> KETAAAKFERQHMDSSTSAASSSNYCNQMMKSRNLTKDRCKPVNTFVHESLADVQAVCSQKNVACKNGQT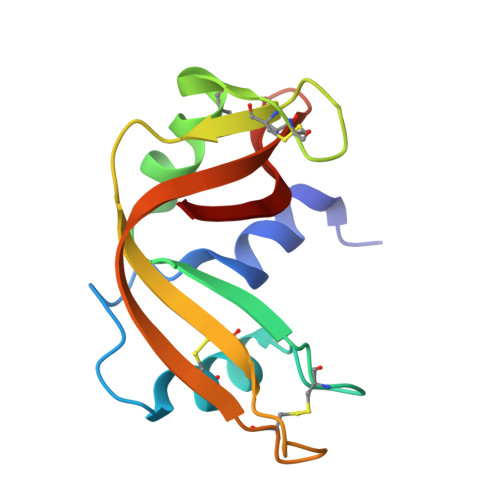NCYQSYSTMSITDCRETGSSKLPNCAYKTTQANKHIIVACEGNPYVPVHFDASV>MHHHHHHSIEGRPHMDFKNINLGIFGHIDHGKTTLSKVLTEIASTSAHDKLPESQKRGITIDIGFSAFKLENYRITLVDAPGHADLIRAVVSAADIIDLALIVVDAKEGPKTQTGEHMLILDHFNIPIIVVITKSDNAGTEEIKRTEMIMKSILQSTHNLKNSSIIPISAKTGFGVDELKNLIITTLNNAEIIRNTESYFKMPLDHAFPIKGAGTVVTGTINKGIVKVGDELKVLPINMSTKVRSIQYFKESVMEAKAGDRVGMAIQGVDAKQIYRGCILTSKDTKLQTVDKIVAKIKISDIFKYNLTPKMKVHLNVGMLIVPAVAVPFKKVTFGKTEENIILNEVISGNECYCAFELEEKVLAEVGDRVLITRLDLPPTTLRICGHGLIEEFKPIKDLNIKKEVLREGKVKIDKGRTVIDGLAQSKVAAEKLIGEEISIEGKDIVGKI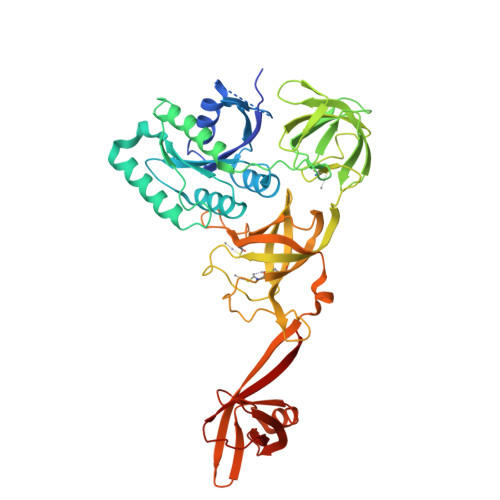KGTFGTKGLLTAEFSGNVENRDKVILNRLRRWG[4x]> KIKDPKILGIDPNVTQYTGYLDVEDEDKHFFFWTFESRNDPAKDPVILWLNGGPGCSSLTGLFFALGPSSIGPDLKPIGNPYSWNSNATVIFLDQPVNVGFSYSGSSGVSNTVAAGKDVYNFLELFFDQFPEYVNKGQDFHIAGASYAGHYIPVFASEILSHKDRNFNLTSVLIGNGLTDPLTQYNYYEPMACGEGGEPSVLPSEECSAMEDSLERCLGLIESCY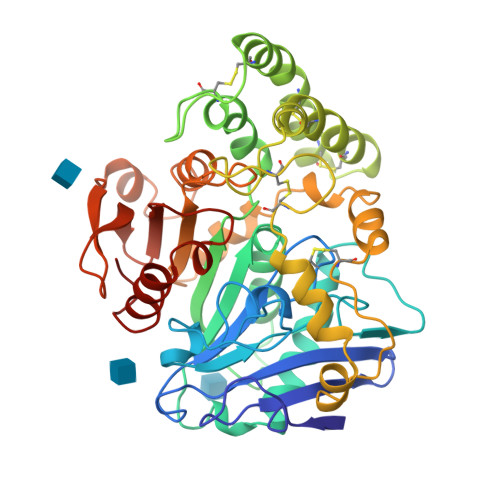DSQSVWSCVPATIYCNNAQLAPYQRTGRNVYDIRKDCEGGNLCYPTLQDIDDYLNQDYVKEAVGAEVDHYESCNFDINRNFLFAGDWMKPYHTAVTDLLNQDLPILVYAGDKDFICNWLGNKAWTDVLPWKYDEEFASQKVRNWTASITDEVAGEVKSYKHFTYLRVFNGGHMVPFDVPENALSMVNEWIHGGFSL> GPEAADIRVLRGHQLSITCLVVTPDDSAIFSAAKDCSIIKWSVESGRKLHVIPRAKKGAEGKPPGHSSHVLCMAISSDGKYLASGDRSKLILIWEAQSCQHLYTFTGHRDAVSGLAFRRGTHQLYSTSHDRSVKVWNVAENSYVETLFGHQDAVAALDALSRECCVTAGGRDGTVRVW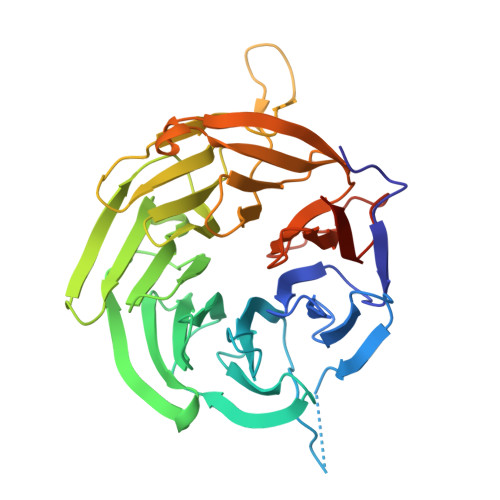KIPEESQLVFYGHQGSIDCIHLINEEHMVSGADDGSVALWGLSKKRPLALQREAHGLRGEPGLEQPFWISSVAALLNTDLVATGSHSSCVRLWQCGEGFRQLDLLCDIPLVGFINSLKFSSSGDFLVAGVGQEHRLGRWWRIKEARNSVCIIPLRRVPVPPAAGS>[4x]STPSIVIASAARTAVGSFNGAFANTPAHELGATVISAVLERAGVAAGEVNEVILGQVLPAGEGQNPARQAAMKAGVPQEATAWGMNQLCGSGLRAVALGMQQIATGDASIIVAGGMESMSMAPHCAHLRGGVKMGDFKMIDTMIKDGLTDAFYGYHMGTTAENVAKQW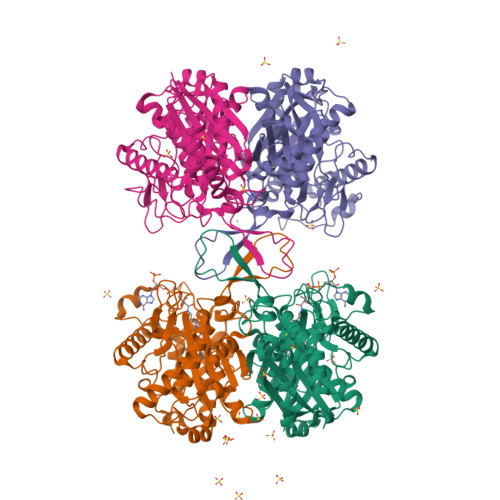QLSRDEQDAFAVASQNKAEAAQKDGRFKDEIVPFIVKGRKGDITVDADEYIRHGATLDSMAKLRPAFDKEGTVTAGNASGLNDGAAAALLMSEAEASRRGIQPLGRIVSWATVGVDPKVMGTGPIPASRKALERAGWKIGDLDLVEANEAFAAQACAVNKDLGWDPSIVNVNGGAIAIGAPIGASGARILNTLLFEMKRRGARKGLATLCIGGGMGVAMCIESL> GSHMRVQVSGMSDETTWHTLKDHLRQAGEVTFCKV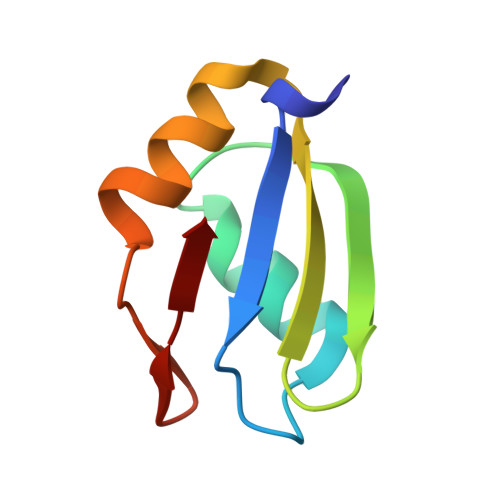FSGGRAVVEFVTPEDAARAITELQASELEGATLFLR> MFKAQATFSRYSAAVSLLLLFSGAAQAAPQSITTLPLQPDGENRWRLPAGEYQGQFTIEQPMQLRCEPGAVIQSQGQGSSLLISAPDVLVEGCTLYEWGSDLTAMDSAVFILPAAERAQISNNRMRGPGFGVFVDGTRDVQVIGNEIDGDAGVRSQDRGNGIHLFAVSGARVLHNHVRNARDGIYIDTSNGNHLEGNVIEDVRYGVHYMFANENSLIDNVTRRTRTGYALMQSRKLTVTGNRSEQDQNYGILMNYITYSTITGNFVSDVQRGDTGGDSMISGGEGKALFIYNSLFNTIENNHFEKSSLGIHLTAGSEDNRISGNAFVGNQQQVKYVASRTQEWSVDGRGNYWSDYLGWDRNNDGLGDIAYE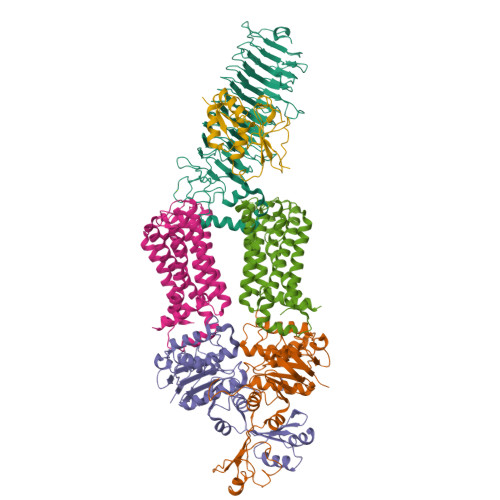PNDNVDRLLWLYPQVRLLMNSPSIEVLRWVQRAFPVIKSPGVQDSHPLMKLPTEKLLTEKQEPTS;>[2x]MNAVEIQGVSQRYGSMTVLHDLNLNLGEGEVLGLFGHNGAGKTTSMKLILGLLSPSEGQVKVLGRAPNDPQVRRQLGYLPENVTFYPQLSGRETLRHFARLKGAALTQVDELLEQVGLAHAADRRVKTYSKGMRQRLGLAQALLGEPRLLLLDEPTVGLDPIATQDLYLLIDRLRQRGTSIILCSHVLPGVEAHINRAAILAKGCLQAVGSLSQLRAEAGLPVRIRASGISERDSWLQRWTDAGHSARGLSESSIEVVAVNGHKLVLLRQLLGEGEPEDIEIHQPSLEDLYRYYMERAGDVRAQEGRL;>[2x]MNQVWNIARKELSDGLRNRWLLAISLLFAVLAVGIAWLGAAASGQLGFTSIPATIASLASLATFLMPLIALLLAYDAIVGEDEGGTLMLLLTYPLGRGQILLGKFVGHGLILALAVLIGFGCAALAIALLVEGVELGMLFWAFGRFMISSTLLGWVFLAFAYVLSGKVNEKSSAAGLALGVWFLFVLVFDLVLLALLVLSEGKFNPELLPWLLLLNPTDIYRLINLSGFEGSGSAMGVLSLGADLPVPAAVLWLCLLAWIGVSLLLAYAIFRRRLT;> MNALHRIGAGTLLAVLLAFGLTGCGEKEEVQQSLEPVAFHDSDECHVCGMIITDFPGPKGQAVEKRGVKKFCSTAEMLGWWLQPENRLLDAKLYVHDMGRSVWEKPDDGHLIDATSAYYVVGTSLKGAMGASLASFAEEQDAKALAGMHGGRVLRFEEIDQALLQEAASMQHGGMHDHAPNGAHNAHAGH>[2x]MSPRSRLLASSLRGGLLLRPCSARRSTLLNPSPSPLRKAIFHTTSLRAFKNLAEIATSSKEDASSLKPKGKPSPPGDPLATIEKTAAEQRRADWAIIKQMSRYLWPKDSWSDKARVLLALSLLVGGKVLNVHVPFYFREIIDRLNIDVAAVGGTVSAVAGAVIFAYGASRIGAVVSQELRNAVFSSVAQKAIRRVATQTFGHLLNLDLSFHLSKQTGGLTRAIDRGTKGISYLLTSMVFHIVPTALEIGMVCGILTYQFGWEFAAITAATMAAYTAFTITTTAWRTKFRRQANAADNAASTVAVDSLINYEAVKYFNNEAYEIARYDKALQAYERSSIKVATSLAFLNSGQNIIFSSALTLMMWLGARGVLAGDLSVGDLVLINQLVFQLSVPLNFLGSVYRELRQSLLDMETLFDLQKVNVTIREAPNAKPLALPKGGEIRFENVTFGYYPDRPILRNLSLTIPAGKKVAVVGPSGCGKSTLLRLLFRSYDPQQGKIFIDDQDIKSVTLESLRKSIGVVPQDTPLFNDTVELNIRYGNVNATQEQVIAAAQKAHIHEKIISWPHGYQTRVGERGLMISGGEKQRLAVSRLILKDPPLLFFDQATSALDTHTEQALMANINEVVKEKKRTALFVAHRLRTIYDADLIIVLKEGVVVEQGSHRELMERDGVYAELWMAQEMLHQGEAAEEPAEGEKAEEKK

Previous studies suggest mitochondrial ABCB7-type exporters are involved in maturation of cytosolic iron-sulfur proteins. Here, we report a series of cryo-electron microscopy structures of a eukaryotic homolog of human ABCB7, CtAtm1, determined at average resolutions ranging from 2.8 to 3.2 Å, complemented by functional characterization and molecular docking in silico. We propose that CtAtm1 accepts delivery from glutathione-complexed iron-sulfur clusters. As anticipated, the architecture of CtAtm1 harbors the classical ABC-fold, packing into a homodimer with six transmembrane segments (TM1–TM6) in each monomer.

How then do [2Fe-2S](GS)4 clusters associate with Atm1 proteins for transport? Interestingly, the 3.2 Å map obtained from the above-mentioned E603Q sample in the presence of the cluster provided a distinct structure, CtAtm1inw-opn-occl (RMSD to CtAtm1inw-opn 1.83 Å). As such, the conformation is reminiscent of cargo-bound ScAtm1, AtAtm3 and NaAtm1 (PDB-IDs 4MYH3,277N5929 and 4MRS3, RMSD 2.6, 2.0, and 2.0 Å, respectively). Indeed, the presence of additional cryo-EM density is detected, coordinated by residues in immediate vicinity of N395, namely R285, R289 of TM4, N348, Q351 of TM5, and S399 of TM6. These coincide with certain of the residues in the mutations (R285A/Q351A and R289A/R402A/Q351A) that display decreased cluster binding and lower iron content, further supportive of the notion that they partake in cluster cargo binding. However, the inner gate is substantially reconfigured in the shift from the inward-facing open states to the CtAtm1inw-opn-occl conformation, reorienting the N395 and F396 pairs, first pointing toward and away from the cavity, respectively, and then vice versa. As no GSH or GSSG was supplemented to the sample, we interpret this feature as a part of the cluster or even a complete cluster with one flexible half; however, conservatively modeled as two GSH molecules. Moreover, molecular docking of [2Fe-2S](GS)4 guided by the cryo-EM density suggests that binding of the entire cluster is possible at this location in the CtAtm1inw-opn-occl conformation. Next, the cargo is recruited to conserved motifs of the binding pocket, coupled to initiation of occlusion and perhaps nucleotide binding, as observed in the partially occluded CtAtm1inw-occl structure. Our data are inconclusive regarding the nature of the bound cargo because only parts of the cluster are detected, although flexibility may partly explain this observation.>SEFSRHSEKIAIRDFQVGDLVLIILDERHDNYVLFTVSPTLYFLHSESLPALDLKPGEGASGASRRPWVLGKVMEKEYCQAKKAQNRFKVPLGTKFYRVKAVSWNKKV[2x];>[2x]SSEDSFVEIRMAE

As a core molecular machinery in mammalian autophagy, the ULK complex is composed of a serine–threonine ULK1/2 kinase, ATG13, ATG101, and FIP200 (also named as RB1CC1), and functions as a master regulator in the initiation of autophagy under the nutrient deprivation condition by linking the upstream nutrient sensors with the downstream autophagy machines. The ULK complex initiates the autophagosome formation, and has recently been implicated in selective autophagy by interacting with autophagy receptors through its FIP200 subunit. Here, we discover that the interactions of FIP200 Claw domain with autophagy receptors CCPG1 and Optineurin can be regulated by the phosphorylation in their respective FIP200-binding regions. In all, our findings uncover a general and phosphoregulatable binding mode shared by many autophagy receptors to interact with FIP200 Claw for autophagosome biogenesis, and are valuable for further understanding the molecular mechanism of selective autophagy.

Consistently, using quantitative fluorescence spectroscopy-based assays, we demonstrated that a 13-residue synthetic S177-phosphorylated Optineurin LIR peptide (‘SSEDpSFVEIRMAE’, referred to as p-Optineurin LIR) can directly bind to FIP200 Claw with a Kd value of ~12 μM, which is ~27-fold stronger than that of the un-phosphorylated Optineurin LIR peptide (Kd ~307 μM). To further uncover the detailed interaction mode between FIP200 Claw and p-Optineurin LIR, we also determined the high-resolution crystal structure of the FIP200 Claw/p-Optineurin LIR complex. As expected, the structure of the FIP200 Claw/p-Optineurin LIR complex is composed of a symmetric FIP200 Claw dimer and two p-Optineurin LIR molecules, each of which mainly forms a short β-strand and directly packs with the β4-strand of FIP200 Claw domain in an anti-parallel fashion. Particularly, the aromatic side chain of Optineurin F178 occupies the LHP of FIP200 Claw, and forms a unique cation-π interaction with the positively charged FIP200 R1584 residue. Meanwhile, the hydrophobic side chains of V179 and I181 pack against the aliphatic side chain of K1568 and the SHG of FIP200, respectively. Moreover, the backbone groups of phosphorylated S177 (p-S177), V179, and I181 form four strong backbone hydrogen bonds with the K1568, Q1566, and Y1564 residues of FIP200. Similar to that of p-CCPG1 FIR2 in binding to FIP200 Claw, the highly positively charged K1569 and R1573 residues decorated around the LHP of FIP200 Claw are neutralized by three negatively charged E175, D176, and p-S177 residues from p-Optineurin LIR. However, in contrast to that of p-CCPG1 FIR2, the phosphate group of the acidic p-S177 preceding the crucial hydrophobic residue that occupies the LHP of FIP200 Claw is coupled with the FIP200 R1573 residue by forming two specific salt bridges and one hydrogen bond, while the side-chain carboxyl group of Optineurin D176 forms a salt bridge with the side chain of K1569 from FIP200.>[4x]GSAKDPMKKIGFIGLGNMGLPMSKNLVKSGYTVYGVDLNKEAEASFEKEGGIIGLSISKLAETCDVVFTSLPSPRAVEAVYFGAEGLFENGHSNVVFIDTSTVSPQLNKQLEEAAKEKKVDFLAAPVSGGVIGAENRTLTFMVGGSKDVYEKTESIMGVLGANIFHVSEQIDSGTTVKLINNLLIGFYTAGVSEALTLAK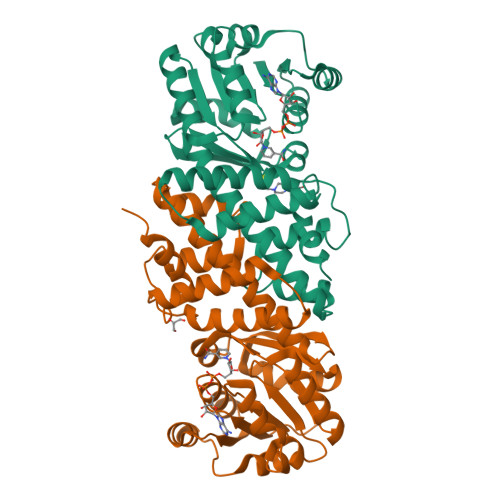KNNMDLDKMFDILNVSYGQSRIYERNYKSFIAPENYEPGFTVNLLKKDLGFAVDLAKESELHLPVSEMLLNVYDEASQAGYGENDMAALYKKVSEQLISNQK>TYTISIRVYQTTPKGFFRPVERTNWKYANGGTWDEVRGEYVLTMGGSGTSGSLRFVSSDTDESFVATFGVHNYKRWCDIVTNLTNEQTALVINQEYYGVPIRDQARENQLTSYNVANAKGRRFAIEYTVTEGDNLKANLIIG[2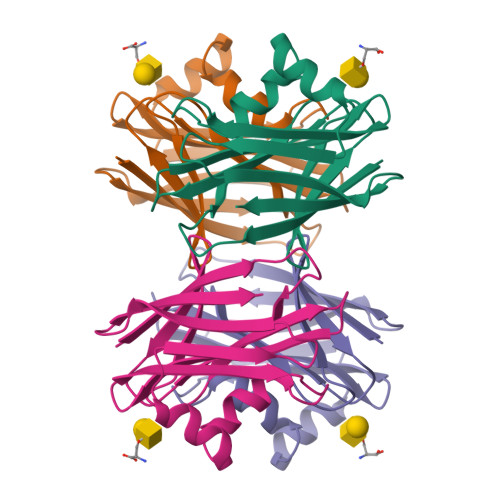x]RING family ubiquitin ligases (E3s) employ the RING domain to recruit the E2 thioester ubiquitin (E2∼Ub) intermediate to catalyze the transfer of ubiquitin (Ub) to substrates. A cationic Arg linchpin (LP) residue in the RING domain plays a key role in stabilizing the interface with E2∼Ub, but the identity of the LP residue varies across E3s. Notably, the position of a cationic Arg residue in the RING domain is conserved in most structures of RING E3/E2∼UbD complexes, where the Arg side chain forms a network of hydrogen bonds with UbD and E2 to stabilize the closed E2∼UbD conformation. We chose the RING domain of RNF38 to use as a model monomeric RING with a native LPArg.

RNF38RING has been crystallized in complex with UBE2D2−Ub previously, yet no high-resolution crystal structure exists of the RNF38RING in isolation. To establish whether Arg454, the native LP residue in RNF38, is constrained by other residues in the absence of E2∼Ub, we determined the structure of RNF38RING to 1.2 Å. RNF38RING adopts a similar structure to that seen in the RNF38RING-UBE2D2–Ub complex (r.m.s. deviation of 0.58 Å for 64 Cα atoms). The location of LPArg within the RNF38 RING domain remains unchanged, with its side chain adopting a slightly different orientation, most likely as a consequence of crystal packing. The observed electron density is well defined in the region, and the conformation of Arg454 is clear, with a B-factor of 17.5 Å2 compared with the overall average B-factor of 18.9 Å2. Briefly, the structure of RNF38 comprises a three-stranded β-sheet, sandwiched between a β-loop–β-motif and an α-helix. All RING domains have a set of conserved Cys and His residues that coordinate two structural Zn2+ ions. In addition, there are differences in the C-terminal tail, which facilitates E2 binding in the complex structures, and is not involved in any interactions outside those of crystal packing in the structure of the RING domain alone.

> GSTKADIEQLPSYRFNPNNHQSEQTLCVVCMCDFESRQLLRVLPCNHEFHAKCVDKWLKANRTCPICRADASEVHRDSE>[2x]MHHHHHHLPNITILATGGTIAGGGDSATKSNYTVGKVGVENLVNAVPQLKDIANVKGEQVVNIGSQDM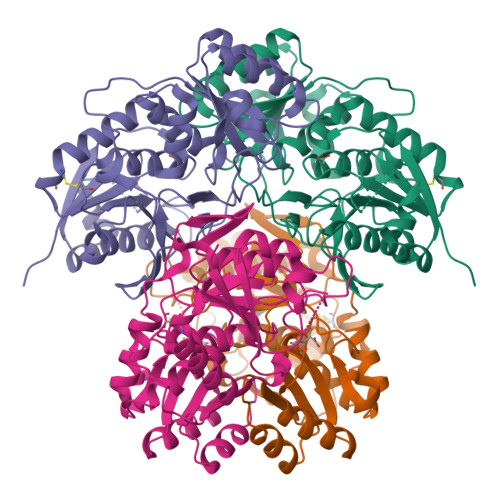NDNVWLTLAKKINTDCDKTDGFVITHGTTTMEETAYFLDLTVKCDKPVVMVGAMRPSTSMSADGPFNLYNAVVTAADKASANRGVLVVMNDTVLDGRDVTTTNTTDVATFKSVNYGPLGYIHNGKIDYQRTPARKHTSDTPFDVSKLNELPKVGIVYNYANASDLPAKALVDAGYDGIVSAGVGNGNLYKSVFDTLATAAKTGTAVVRSSRVPTGATTQDAEVDDAKYGFVASGTLNPQKARVLLQLALTQTKDPQQIQQIFNQY>[2x]MCTAGKDITCKAAVAWEPHKPLSLETITVAPPKAHEVRIKILASGICGSDSSVLKEIIPSKFPVILGHEAVGVVESIGAGVTCVKPGDKVIPLFVPQCGSCRACKSSNSNFCEKNDMGAKTGLMADMTSRFTCRGKPIYNLMGTSTF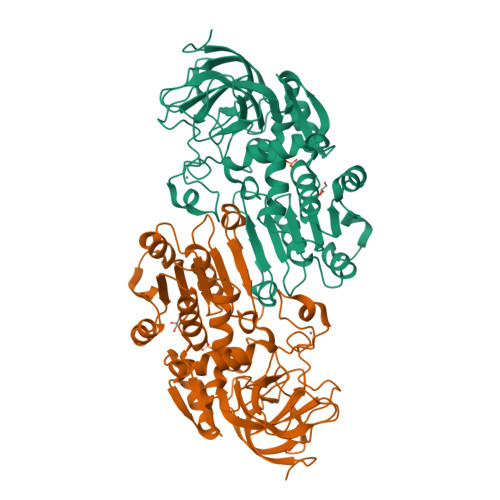TEYTVVADIAVAKIDPKAPLESCLIGCGFATGYGAAVNTAKVTPGSTCAVFGLGGVGFSAIVGCKAAGASRIIGVGTHKDKFPKAIELGATECLNPKDYDKPIYEVICEKTNGGVDYAVECAGRIETMMNALQSTYCGSGVTVVLGLASPNERLPLDPLLLLTGRSLKGSVFGGFKGEEVSRLVDDYMKKKINVNFLVSTKLTLDQINKAFELLSSGQGVRSIMIY>[16x]VLPENMKRYMGRDAQRMNILAGRIIAETVRSTLGP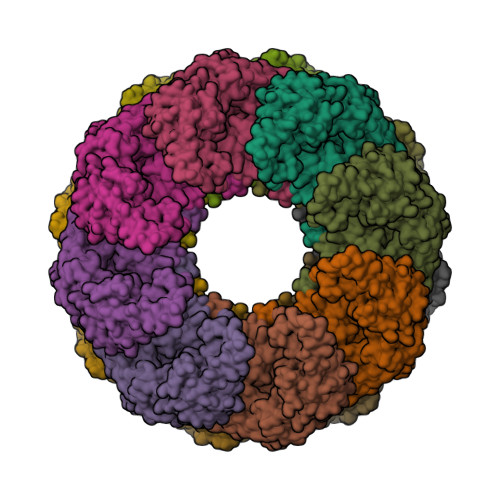KGMDKMLVDDLGDVVVTNDGVTILREMSVEHPAAKMLIEVAKTQEKEVGDGTTTAVVVAGELLRKAEELLDQNVHPTIVVKGYQAAAQKAQELLKTIACEVGAQDKEILTKIAMTSITGKGAEKAKEKLAEIIVEAVSAVVDDEGKVDKDLIKIEKKSGASIDDTELIKGVLVDKERVSAQMPKKVTDAKIALLNCAIEIKETETDAEIRITDPAKLMEFIEQEEKMLKDMVAEIKASGANVLFCQKGIDDLAQHYLAKEGIVAARRVKKSDMEKLAKATGANVITNIKDLSAQDLGDAGLVEERKISGDSMIFVEECKHPKAVTMLIRGTTEHVIEEVARAVDDAVGVVGCTIEDGRIVSGGGSTEVELSMKLREYAEGISGREQLAVRAFADALEVIPRTLAENAGLDAIEILVKVRAAHASNGNKCAGLNVFTGAVEDMCENGVVEPLRVKTQAIQSAAESTEMLLRIDDVIAAE>MRCVGVGNRDFVEGLSGATWVDVVLEHGGCVTTMAKNKPTLDIELQKTEATQLATLRKLCIEGKITNITTDSRCPTQGEAVLPEEQDQNYVCKHTYVDRGWGNGCGLFGKGSLVTCAKFQCLEPIEGKVVQYENLKYTVIITVHTGDQHQVGNETQGVTAEITPQASTTEAILPEYGTLGLECSPRTGLDFNEMILLTMKNKAWMVHRQWFFDLPLPWASGATTETPTWNRKELLVTFKNAHAKKQEVVVLGSQEGAMHTALTGATEIQNSGGTSIFAGHLKCRLKMDKLELKGMSYAMCTNTFVLKKEVSETQHGTILIKVEYKGEDAPCKIPFSTEDGQGKAHNGRLITANPVVTKKEEPVNIEAEPPFGESNIVIGIGDNALKINWYKKGSSIGKMFEATARGARRMAILGDTAWDFGSVGGVLNSLGKMVHQIFGSAYTALFSGVSWVMKIGIGVLLTWIGLNSKNTSMSFSCIAIGIITLYLGAVVQA[3x];>[3x]SVALAPHVGMGLDTRTQTWMSAEGAWRQVEKV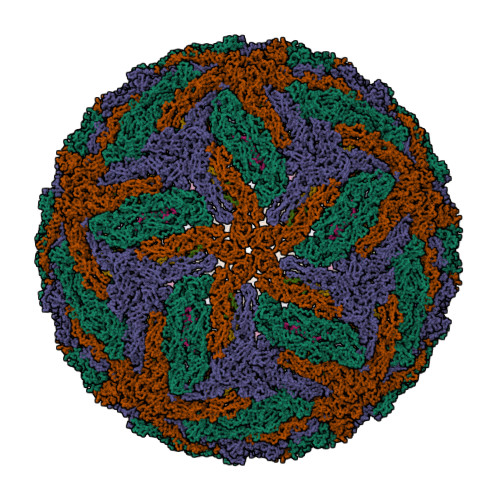ETWALRHPGFTILALFLAHYIGTSLTQKVVIFILLMLVTPSMT>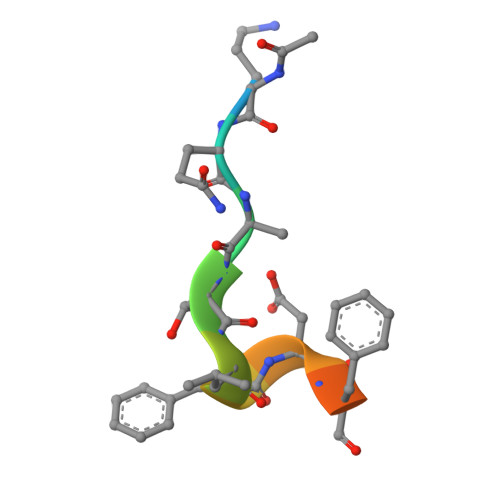 XKQATLFDFLKK>ADPSKDSKAQVSAAEAGITGTWYNQLGSTFI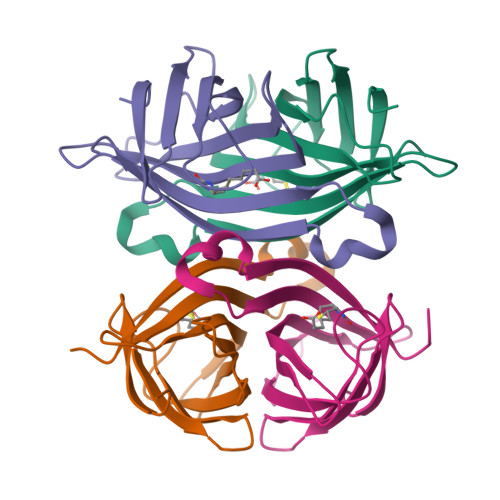VTAGADGALTGTYESAVGNAESRYVLTGRYDSAPATDGSGTALGWTVAWKNNYRNAHSATTWSGQYVGGAEARINTQWLLTSGTTEANAKKSTLVGHDTFTKVKP[4x]> MKLTPK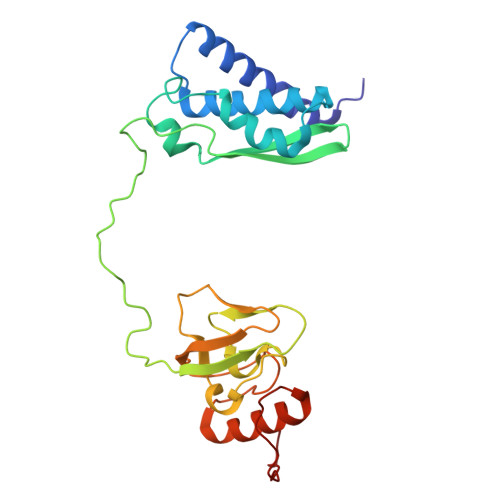ELDKLMLHYAGELAKKRKEKGIKLNYVEAVALISAHIMEEARAGKKTAAELMQEGRTLLKPDDVMDGVASMIHEVGIEAMFPDGTKLVTVHTPIEANGKLVPGELFLKNEDITINEGKKAVSVKVKNVGDRPVQIGSHFHFFEVNRCLDFDREKTFGKRLDIAAGTAVRFEPGEEKSVELIDIGGNRRIFGFNALVDRQADNESKKIALHRAKERGFHGAKSDDNYVKTIKE2-{5-[AMINO(IMINIO)METHYL]-1H-BENZIMIDAZOL-2-YL}PYRIDIN-3-OLATE 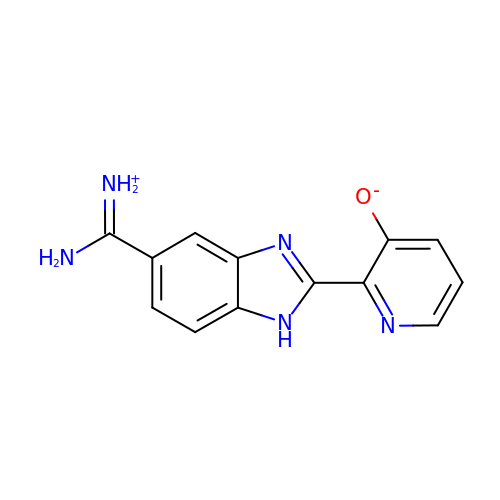| C13 H11 N5 O | FQCDQFDJHSXQKY-UHFFFAOYSA-N>GEIEFIESSKDAGFPVINTPSKTKLEPSVFHQVFEGNKEPAVLRSGDPRLKANFEEAIFSKYIGNVNTHVDEYMLEAVDHYAGQLATLDISTEPMKLEDAVYGTEGLEALDLTTSAGYPYVALGIKKRDILSKKTKDLTKLKECMDKYGLNLPMVTYVKDELRSIEKVAKGKSRLIEASSLNDSVAMRQTFGNLYKTFHLNPGVVTGSAVGCDPDLFWSKIPVMLDGHLIAFDYSGYDASLSPVWFACLKMILEKLGYTHKETNYIDYLCNSHHLYRDKHYFVRGGMPSGCSGTSIFNSMINNIIIRTLMLKVYKGIDLDQFRMIAYGDDVIASYPWPIDASLLAEAGKGYGLIMTPADKGECFNEVTWTNVTFLKRYFRADEQYPFLVHPVMPMKDIHESIRWTK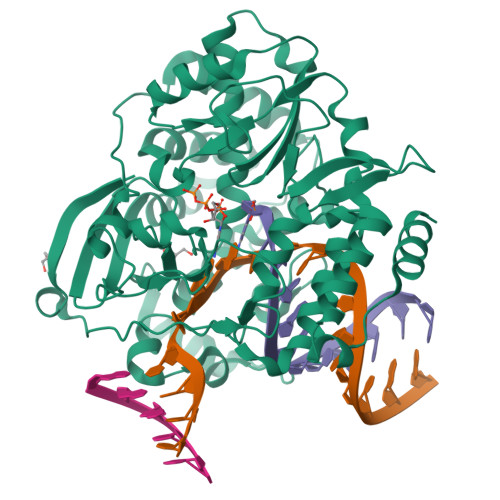DPKNTQDHVRSLCLLAWHNGEHEYEEFIRKIRSVPVGRCLTLPAFSTLRRKWLDSFGSSSHHHHHH[4x]> SEDEEDILARVDLETTRAIAKQMFSSGTVVEVSSDEEGFQGCWFAAKVVEPVGEDKFLVEYRDLREKDGIEPLKEETDFLHIRPPPPRDEDIDFAVGDKINAFYNDGWWVGVVIDGMKHGTVGIYFRQSQEKMRFGRQGLRLHKDWVDGTWQLPLKGGKIKREKTVS

Here, we identify a previously uncharacterized H3K9me2-binding protein, which was named AGD-containing protein 1 (AGDP1). The AGDP1 protein possesses three pairs of tandem AGDs (AGD12, AGD34, and AGD56), all of which can specifically recognize the H3K9me2 mark. Our biochemical and structural studies reveal the molecular basis for the specific recognition of the dual marks H3K4me0 and H3K9me2 by the three tandem AGD cassettes of AGDP1. Our studies identify an H3K9me2-binding protein that regulates heterochromatic DNA methylation and reveal the molecular basis for the specific recognition of H3K9me2 mark, thus establishing an additional linkage between H3K9me2 and heterochromatic DNA methylation.

We also performed structural studies on AGD34 and AGD56 of AtAGDP1. We obtained the free-form structure of AtAGDP1 AGD34. The overall structure of AtAGDP1 AGD34 resembles that of RsAGDP1 AGD12 with all the peptide-binding residues, especially the H3K4me0- and H3K9me2-binding residues, conserved and occupying the same positions. The structure-based sequence alignment of AtAGDP1 and RsAGDP1 tandem AGD cassettes indicates that most of the peptide-interacting residues, especially the H3K4- and H3K9me2-binding residues, are conserved. Intriguingly, all three tandem AGD cassettes (AGD12, AGD34, and AGD56) can specifically bind to the methylated H3K9 mark with preference on H3K9me2, suggesting that a single AGDP1 protein has multiple H3K9me2-binding sites. In contrast, the AtAGD34 and AtAGD56 binds to H3K9me2 about twofold higher than H3K9me1, although the peptide-binding regions are quite conserved. Our in vitro binding data suggest that a single AGDP1 protein possesses three H3K9me2-binding sites and sequence alignment results indicate that the AGD12, AGD34, and AGD56 can each capture an H3K9me2 mark using the same mechanism.> SEFRRQTIRHSTREKDRGPTKATTTKLVYQIFDTFFAEQIEKDDREDKENAFKRRRCGVCEVCQQPECGKCKACKDMVKFGGSGRSKQACQERRCPNMAMKEADDDEEVDDNIPEMPSPKKMHQGKKKKQNKNRISWVGEAVKTDGKKSYYKKVCIDAETLEVGDCVSVIPDDSSKPLYLARVTALWEDSSNGQMFHAHWFCAGTDTVLGATSDPLELFLVDECEDMQLSYIHSKVKVIYKAPSENWAMEGGMDPESLLEGDDGKTYFYQLWYDQDYARFESPPKTQPTEDNKFKFCVSCARLAEMRQKEIPRVLEQLEDLDSRVLYYSATKNGILYRVGDGVYLPPEAFTFNIKLSSPVKRPRKEPVDEDLYPEHYRKYSDYIKGSNLDAPEPYRIGRIKEIFCPKKSNGRPNETDIKIRVNKFYRPENTHKSTPASYHADINLLYWSDEEAVVDFKAVQGRCTVEYGEDLPECVQVYSMGGPNRFYFLEAYNAKSKSFEDPPNHARSPGNKGKGKGKGKGKPKSQACEPSEPEIEIKLPKLRTLDVFSGCGGLSEGFHQAGISDTLWAIEMWDPAAQAFRLNNPGSTVFTEDCNILLKLVMAGETTNSRGQRLPQKGDVEMLCGGPPCQGFSGMNRFNSRTYSKFKNSLVVSFLSYCDYYRPRFFLLENVRNFVSFKRSMVLKLTLRCLVRMGYQCTFGVLQAGQYGVAQTRRRAIILAAAPGEKLPLFPEPLHVFAPRACQLSVVVDDKKFVSNITRLSSGPFRTITVRDTMSDLPEVRNGASALEISYNGEPQSWFQRQLRGAQYQPILRDHICKDMSALVAARMRHIPLAPGSDWRDLPNIEVRLSDGTMARKLRYTHHDRKNGRSSSGALRGVCSCVEAGKACDPAARQFNTLIPWCLPHTGNRHNHWAGLYGRLEWDGFFSTTVTNPEPMGKQGRVLHPEQHRVVSVRECARSQGFPDTYRLFGNILDKHRQVGNAVPPPLAKAIGLEIKLCMLAKA;> GPLGSEAHLYMQVQIVAEDQFCGHQGNDMYDEEKVKYTVFKVLKNSSLAEFVQSLSQTMGFPQDQIRLWPMQARSNGTKRPAMLDNEADGNKTMIELSDNENPWTIFLETVDPELAASGATLPKFDKDHDVMLFLKMYDPKTRSLNYCGHIYTPISCKIRDLLPVMCDRAGFIQDTSLILYEEVKPNLTERIQDYDVSLDKALDELMDGDIIVFQKDDPENDNSELPTAKEYFRDLYHRVDVIFCDKTIPNDPGFVVTLSNRMNYFQVAKTVAQRLNTDPMLLQFFKSQGYRDGPGNPLRHNYEGTLRDLLQFFKPRQPKKLYYQQLKMKITDFENRRSFKCIWLNSQFREEEITLYPDKHGCVRDLLEECKKAVELGEKASGKLRLLEIVSYKIIGVHQEDELLECLSPATSRTFRIEEIPLDQVDIDKENEMLVTVAHFHKEVFGTFGIPFLLRIHQGEHFREVMKRIQSLLDIQEKEFEKFKFAIVMMGRHQYINEDEYEVNLKDFEPQPGNMSHPRPWLGLDHFNKAPKRSRYTYLEKAIKIHN

DNMT1 is an important epigenetic regulator and plays a key role in the maintenance of DNA methylation during DNA replication. USP7 is the first identified and only known deubiquitinase that binds to and stabilizes DNMT1. To explore the molecular mechanism for USP7-mediated stabilization of DNMT1, we determined the crystal structure of human DNMT1 in complex with USP7. Structural and biochemical analyses reveal that the interaction is mainly mediated by the KG linker of DNMT1 and a previously uncharacterized acidic pocket that acts as a substrate-binding site near the C-terminus of USP7.

We next determined the crystal structure of DNMT1 (residues 600–1,600, designated as DNMT1 if not specified) in complex with TUDUSP7 at 2.9 Å resolution. In the complex structure, USP7 binds to the BAH2 domain (lemon) and target recognition domain (TRD) of DNMT1 (green) on two separate interfaces (Interface-1 and Interface-2). In the DNMT1–USP7 structure, TUDUSP7 consist of three separate modules, UBL1–2, UBL3 and UBL4–5, which are connected by two hinge regions flanking UBL3 and collectively adopt an extended conformation. Superposition of the UBL4–5 domains from the two structures results in a separation of the respective UBL1–2 domains by as much as 40 Å. This analysis indicates that complex formation leads to a significant conformational change in TUDUSP7, which primarily occurs at the hinge regions flanking the UBL3 domain. Interface-1 primarily involves the KG linker of DNMT1 (residues 1,109–1,119, designated as KGDNMT1) and an acidic groove on the surface of UBL1–2USP7. Residue K1111DNMT1 snugly inserts into an acidic cave formed by residues E736, D758, E759 and D764 of USP7. Residue K1115DNMT1 binds to the carbonyl oxygen atoms of residues D684 and D762 of USP7. The Interface-2 involves TRDDNMT1 and UBL3USP7, with a buried surface area of 676 Å2. Taken together, the KGDNMT1 (especially residue K1111) and the acidic pocket of the TUDUSP7 on the Interface-1 are important for the interaction between DNMT1 and USP7. An acetylation mimic mutant (DNMT14KQ) or acetylation of four Lysine residues on the KG linker of DNMT1 led to a decrease in its binding affinity to USP7 and a decrease in its protein stability.> SDACVHHIKRRDIVLKWELGEGAFGKVFLAECHNLLPEQDKMLVAVKALKEASESARQDFQREAELLTMLQHQHIVRFFGVCTEGRPLLMVFEYMRHGDLNRFLRSHGPDAKLLAGGEDVAPGPLGLGQLLAVASQVAAGMVYLAGLHFVHRDLATRNCLVGQGLVVKIGDFGMSRDIYSTDYYRVGGRTMLPIRWMPPESILYRKFT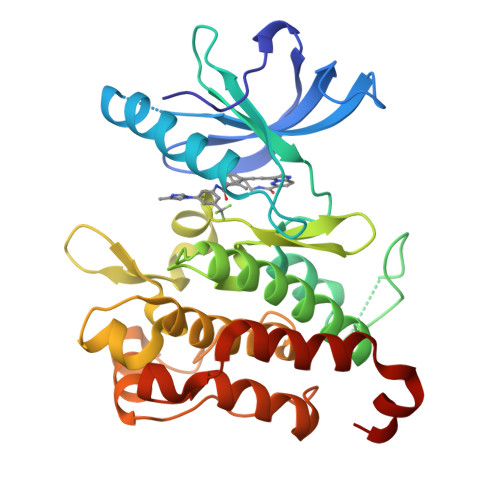TESDVWSFGVVLWEIFTYGKQPWYQLSNTEAIDCITQGRELERPRACPPEVYAIMRGCWQREPQQRHSIKDVHARLQALAQAPPVYLDVLG>GKLPPVYPVTVPILGHIIQFGKSPLGFMQECKRQLKSGIFTINIVGKRVTIVGDPHEHSRFFLPRNEVLSPREVYSFMVPVFGEGVAYAAPYPRMREQLNFLAEELTIAKFQNFVPAIQHEVRKFMAANWDKDEGEINLLEDCSTMIINTACQCLFGEDLRKRLDARRFAQLLAKMESSLIPAAVFLPILLKLPLPQSARCHEARTELQKILSEIIIARKEEEVNKDSSTSDLLSGLLSAVYRDGTPMSLHEVCGMIVAAMFAGQHTSSITTTWSMLHLMHPANVKHLEALRKEIEEFPAQLNYNNVMDEMPFAERCARESIRRDPPLLMLMRKVMADVKVGSYVV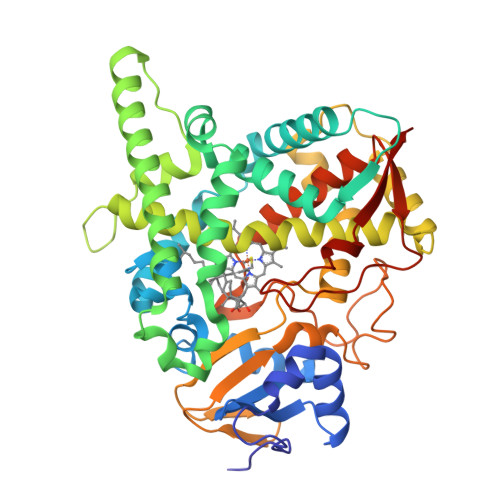PKGDIIACSPLLSHHDEEAFPEPRRWDPERDEKVEGAFIGFGAGVHKCIGQKFGLLQVKTILATAFRSYDFQLLRDEVPDPDYHTMVVGPTASQCRVKYIRRKAAAA[4x]>[2x]NATEIRASVGKMIDGIGRFYIQMCTELKLSDYEGRLIQNSLTIERMVLSAFDTGGPIYRRVDGKWRRELILYDKEEIRRIWRQANNGDDATAGLTHMMIWHSNLNDATYQRTRALVRTGMDPRMCSLMQGSTLPRRSGAAGAAVKGVGTMVMELIRMIKRGINRRTRIAYERMCNILKGKFQTAAQRTMVDQVRESRNPGNAEFEDLIFLARSALILRGSVAHKSCLPACVYGS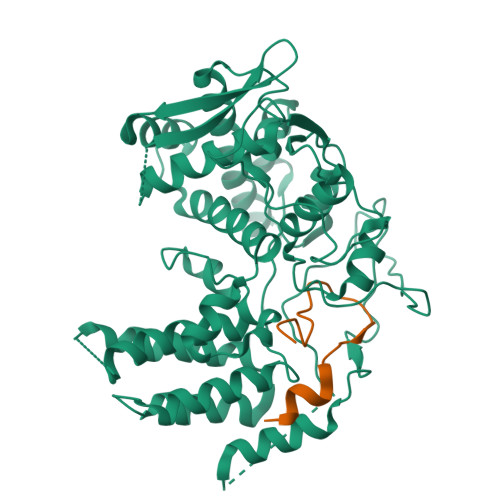AVASGYDFEREGYSLVGIDPFRLLQNSQVYSLIRPNENPAHKSQLVWMACHSAAFEDLRVSSFIRGTKVVPRGKLSTRGVQIASNENMETMESSTLELRSRYWAIRTRSGGNTSDMRTEIIRLMESARPEDVSFQGRGVFELSDEKATSPIVPSFDMSNEGSYFF;>SSGQISIQPTFSVQRNLPFDRPTIMAA[2x]> MNSTHHYEQLIEIFNSCFADEFNTRLIKGDDEPIYLPADAEVPYNRIVFAHGFYASAIHEISHWCIAGKARRELVDFGYWYCPDGRDAQTQSQFEDVEVKPQALDWLFCVAAGYPFNVSCDNLEGDFEPDRVVFQRRVHAQVMDYLANGIPERPARFIKALQNYYYTPELTAEQFPWPEALSLEHHHHHH

A recent study revealed that the β-lysylated Lys34 of EF-P is subsequently hydroxylated at C4(γ) or C5(δ) by YfcM. Although YfcM is structurally different from any other hydroxylation enzymes reported so far, YfcM shares similarity with the ribonuclease YbeY, despite their low sequence homology. Furthermore, the three-histidine motif of YbeY for the coordination of a metal ion is replaced with a putative 2-His-1-carboxylate motif for the coordination of an Fe(II) in YfcM. The structure consists of five α-helices (α1–α5) and a β sheet composed of three β strands (β1–β3).

In order to confirm that an Fe(II) ion is coordinated by the putative 2-His-1-carboxylate motif of YfcM, we prepared crystals of Co(II)-bound YfcM and calculated the anomalous difference Fourier map, using the data set collected at the peak wavelength of the Co K-shell absorption edge (1.6049 Å). The Co(II) ion has an ionic radius similar to that of an Fe(II) ion and can adopt the geometry of an octahedral complex together with six ligands, similar to an Fe(II) ion. Therefore, a Co(II) ion often binds to the 2-His-1-carboxylate motif in a manner that mimics an Fe(II) ion. Furthermore, a Co(II) ion occupies an Fe(II) ion-coordinating site more stably than an Fe(II) ion, because an Fe(II) ion is easily air-oxidized to an Fe(III) ion, thus changing its ionic radius. The resultant electron density map clearly exhibited a strong Co(II) peak at the metal-coordinating site, indicating that a Co(II) ion can be coordinated by His59, His63 and Glu98. In this structure, six atoms participate in the Co(II) ion coordination (nitrogen atoms (NEs) of His59 and His63, two oxygen atoms (OEs) of Glu98 and two oxygen atoms of two water molecules; distances from the Co(II) ion are summarized in Supplementary Table S5), which may mimic the Fe(II) ion coordination. Therefore, our data suggested that His59, His63 and Glu98 of YfcM form the putative 2-His-1-carboxylate motif for the coordination of an Fe(II) ion, as in the active sites of non-heme iron enzymes. Our atomic absorption spectrometry and X-ray crystallographic analyses confirmed the interaction of an Fe ion with YfcM, and the binding of a Co(II) ion to the putative 2-His-1-carboxylate motif of YfcM in a manner mimicking an Fe(II) ion.> MEFMRVERVLLKDYTTLGVGGPAELWTVETRE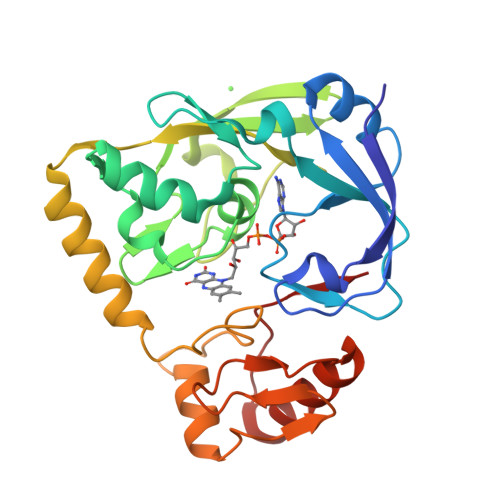ELKRATEAPYRVLGNGSNLLVLDEGVPERVIRLAGEFQTYDLKGWVGAGTLLPLLVQEAARAGLSGLEGLLGIPAQVGGAVKMNAGTRFGEMADALEAVEVFHDGAFHVYCPEELGFGYRKSHLPPGGIVTRVRLKLKERPKEEILRRMAEVDRARKGQPKRKSAGCAFKNPPGQSAGRLIDERGLKGLRVGDAMISLEHGNFIVNLGQARAKDVLELVRRVQEELPLELEWEVWP> XNEGDAAKGEKEFNKCKAC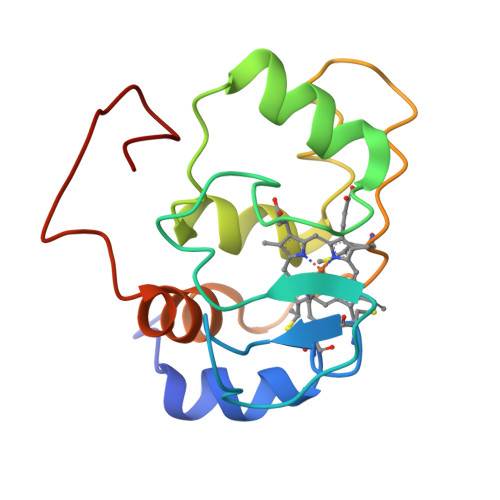HMIQAPDGTDIKGGKTGPNLYGVVGRKIASEEGFKYGEGILEVAEKNPDLTWTEANLIEYVTDPKPLVKKMTDDKGAKTKMTFKMGKNQADVVAFLAQDDPDAXXXXXXXXXXXXX> MSSRKSKSNSLIHTECLSQVQRILRERFCRQSPHSNLFGVQVQYKHLSELLKRTALHGESNSVLIIGPRGSGKTMLINHALKELMEIEEVSENVLQVHLNGLLQINDKIALKEITRQLNLENVVGDKVFGSFAENLSFLLEALKKGDRTSSCPVIFILDEFDLFAHHKNQTLLYNLFDISQSAQTPIAVIGLTCRLDILELLEKRVKSRFSHRQIHLMNSFGFPQYVKIFKEQLSLPAEFPDKVFAEKWNENVQYLSEDRSVQEVLQKHFNISKNLRSLHMLLMLALNRVTASHPFMTAVDLMEASQLCSMDSKANIVHGLSVLEICLIIAMKHLNDIYEEEPFNFQMVYNEFQKFVQRKAHSVYNFEKPVVMKAF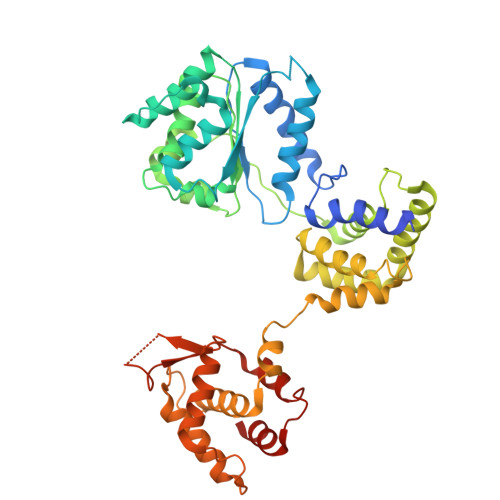EHLQQLELIKPMERTSGNSEREYQLMKLLLDNTQIMNALQKYPNCPTDVRQWATSSLSWL>[2x]MDQWSMLRHFDHITKDYHDHIAEISAKLVAIMDSL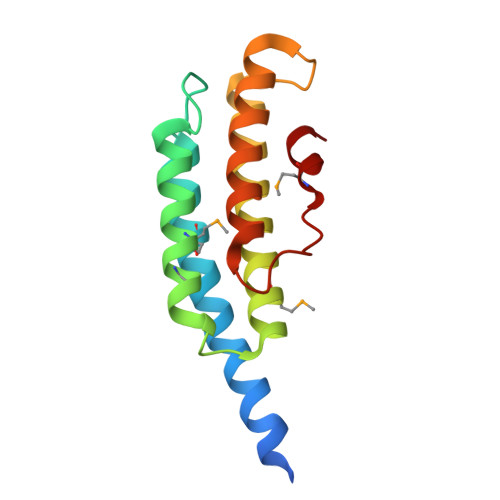FDKLLSKYEVKAPVPSPCFRNICKQMTKMHEAIFDLLPEEQTQMLFLRINASYKLHLKKQLSHLNVINDGGPQNGLVTADVAFYTGNLQALKGLKDLDLNMAEIWE> N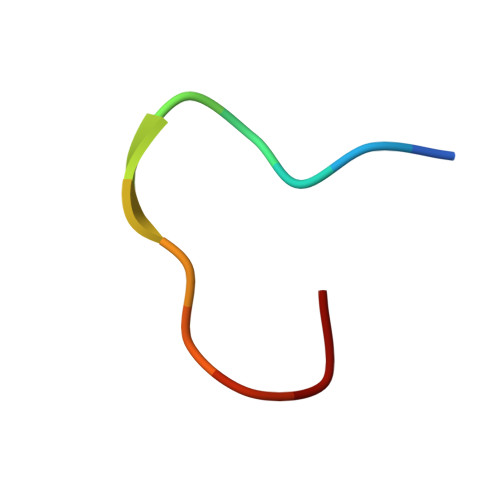PPPPGFIMHGN>[2x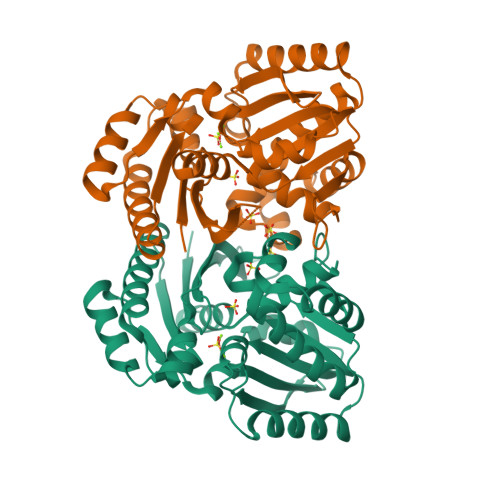]GPLGSMEKVHYAAIDVGSNAVRLLIKCVNSEGMEEPLSKVLIMRVPIRLGEDSFTKGYIGEEKADNMVRLMRAYNEMMQIYRVKDYRACATSAMRDASNAEAVIAQIREKTGIHIDIIDGDEEARLVSDNHIEQIISDGGNYIYLDVGGGSTELTLFSDTHIKHSQSFDIGTVRLLSEKVRPYVREAFRSELMAITKEYTDITIIGTGGNINRLVRLSGSDRGSSRYSIMPVEALHKTYDLLKPISTEERMVRFHLKPDRADVIIPAAEIFLEVADITGAKTIIAPIVGLADGIIEDLYIRHQSRPS> MKLYSLSVLYKGEAKVVLLKAAYDVSSFSFFQRSSVQEFM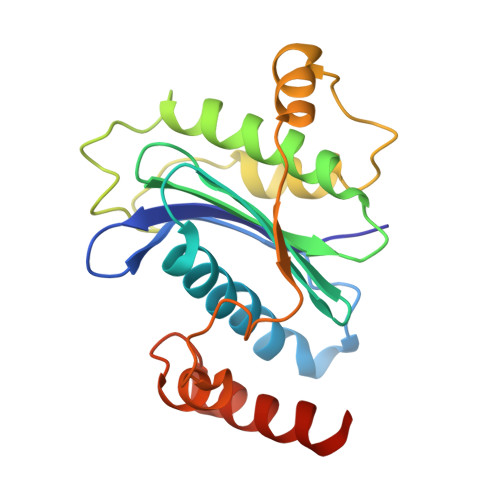TFTSQLIVERSSKGTRASVKEQDYLCHVYVRNDSLAGVVIADNEYPSRVAFTLLEKVLDEFSKQVDRIDWPVGSPATIHYPALDGHLSRYQNPREADPMTKVQAELDETKIILHNTMESLLERGEKLDDLVSKSEVLGTQSKAFYKTARKQNSCCAIM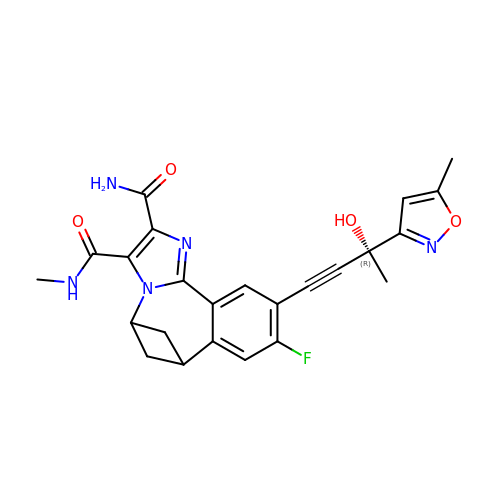(5s,7s)-9-fluoro-10-[(3R)-3-hydroxy-3-(5-methyl-1,2-oxazol-3-yl)but-1-yn-1-yl]-N~3~-methyl-6,7-dihydro-5H-5,7-methanoimidazo[2,1-a][2]benzazepine-2,3-dicarboxamide | C24 H22 F N5 O4 | GFVXWRXUSFUWQS-QWJLCTJOSA-N>[4x]GSHMNKLVVLGSVNADHVLQVPSFPRPGETLHGRNYQVIP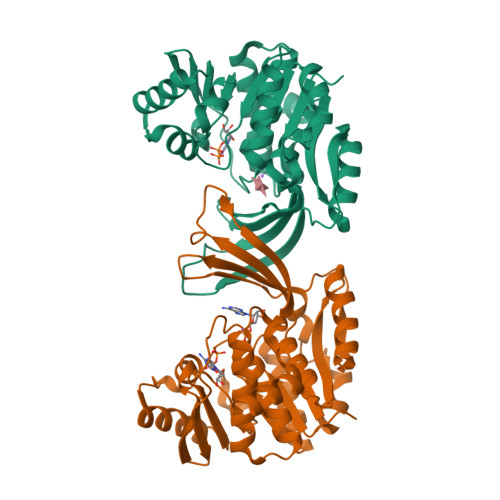GGKGANQAVAAARMQADVGFIACVGDDSFGINIRESFKLDGINTAGVKLQPNCPTGIAMIQVSDSGENSICISAEANAKLTAAAIEPDLAAIRDARYLLMQLETPLDGILKAAQEAKTAKTNVILNPAPARELPDELLKCVDLITPNETEAEVLTGITVYDDSSAQQAADALHCKGIEIVIITLGSKGVWLSQNGRGQRIPGFVVKATDTTAAGDTFNGALVTGLLQEMPLESAIKFAHAAAAISVTRFGAQTSIPTRAEVEAFLAEHS N-{6-(CYCLOPROPYLMETHOXY)-7-METHOXY-2-[6-(2-METHYLPROPYL)-5-OXO-3,4,5,6-TETRAHYDRO-2,6-NAPHTHYRIDIN-2(1H)-YL]QUINAZOLIN-4-YL}-2,2,2-TRIFLUOROETHANESULFONAMIDE 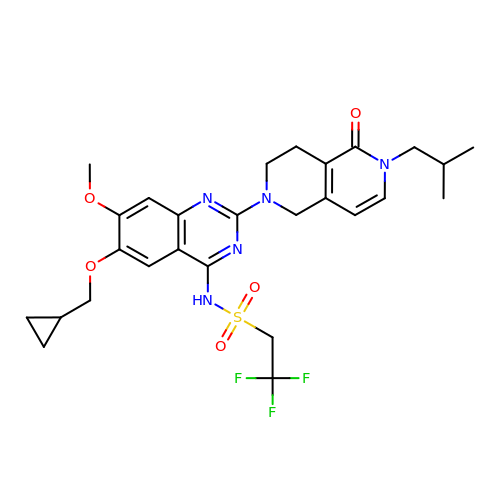| C27 H32 F3 N5 O5 S | HFFZUKFYGADHSF-UHFFFAOYSA-N>ATKVAVAGASGYAGGEILRLLLGHPAYADGRLRIGALTAATSAGSTLGEHHPHLTPLAHRVVEPTEAAVLGGHDAVFLALPHGHSAVLAQQLSPETLIIDCGADFRLTDAAVWERFYGSSHAGSWPYGLPELPGARDQLRGTRRIAVPGCYPTAALLALFPALAADLIEPAVTVVAVSGTSGAGRAATTDLLGAEVIGSARAYNIAGVHRHTPEIAQGLRAVTDRDVSVSFTPVLIPASRGILATCTARTRSPLSQLRAAYEKAYHAEPFIYLMPEGQLPRTGAVI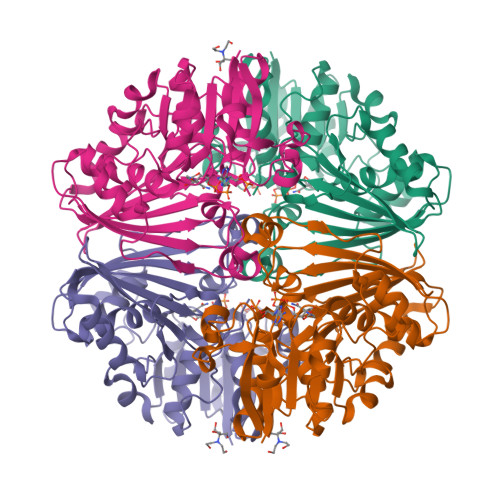GSNAAHIAVAVDEDAQTFVAIAAIDNLVKGTAGAAVQSMNLALGWPETDGLSVVGVAP[4x]>[5x]ASLAADTPTACCFSYTSRQIPQNFIADYFETSSQCSKPGVIFLTKRSRQVCADPS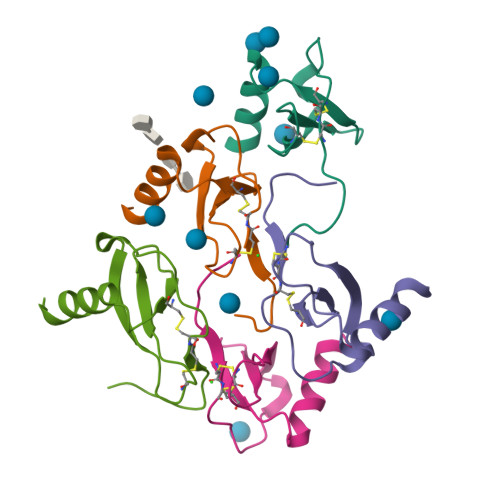EEWVQKYVSDLELSA2,5-diethyl-1-methyl-4-sulfamoyl-pyrrole-3-carboxylic acid | C10 H16 N2 O4 S | 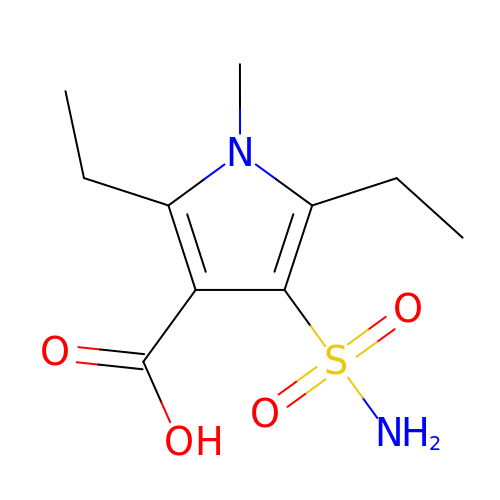XSESKJZGUOEQOI-UHFFFAOYSA-N> MNSPISPIETVPVKLKPGMDGPKVKQWPLTEEKIKALVEICTEMEKEGKISKIGPENPYNTPVFAIKKKDSTKWRKLVDFRELNKRTQDFWEVQLGIPHPAGLKKKKSVTVLDVGDAYFSVPLDEDFRKYTAFTIPSINNETPGIRYQYNVLPQGWKGSPAIFQSSMTKILEPFRKQNPDIVICQYMDDLYVGSDLEIGQHRTKIEELRQHLLRWGLTTPDKKHQKEPPFLWMGYELHPDKWTVQPIVLPEKDSWTVNDIQKLVGKLNWASQIYPGIKVRQLCKLLRGTKALTEVIPLTEEAELELAENREILKEPVHGVYYDPSKDLIAEIQKQGQGQWTYQIYQEPFKNLKTGKYARMRGAHTNDVKQL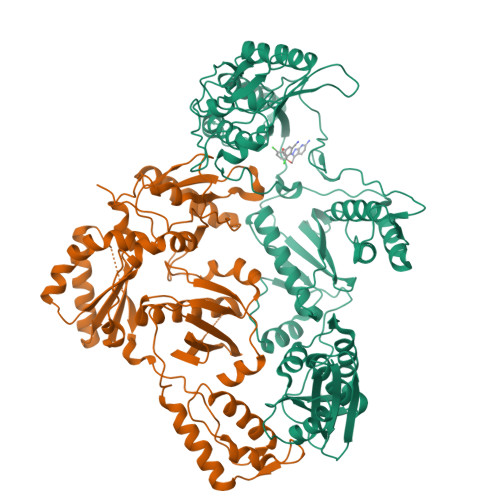TEAVQKITTESIVIWGKTPKFKLPIQKETWETWWTEYWQATWIPEWEFVNTPPLVKLWYQLEKEPIVGAETFYVDGAANRETKLGKAGYVTNRGRQKVVTLTDTTNQKTELQAIYLALQDSGLEVNIVTDSQYALGIIQAQPDQSESELVNQIIEQLIKKEKVYLAWVPAHKGIGGNEQVDKLVSAGIRKVL;> MNSPISPIETVPVKLKPGMDGPKVKQWPLTEEKIKALVEICTEMEKEGKISKIGPENPYNTPVFAIKKKDSTKWRKLVDFRELNKRTQDFWEVQLGIPHPAGLKKKKSVTVLDVGDAYFSVPLDEDFRKYTAFTIPSINNETPGIRYQYNVLPQGWKGSPAIFQSSMTKILEPFRKQNPDIVICQYMDDLYVGSDLEIGQHRTKIEELRQHLLRWGLTTPDKKHQKEPPFLWMGYELHPDKWTVQPIVLPEKDSWTVNDIQKLVGKLNWASQIYPGIKVRQLCKLLRGTKALTEVIPLTEEAELELAENREILKEPVHGVYYDPSKDLIAEIQKQGQGQWTYQIYQEPFKNLKTGKYARMRGAHTNDVKQLTEAVQKITTESIVIWGKTPKFKLPIQKETWETWWTEYWQATWIPEWEFVNTPPLVKLWYQLEKEPIVGAETF A glutamine synthetase-like (GS-like) enzyme (NpaA1) initiates 1NA glutamylation, and this enzyme exhibits a broad substrate selectivity toward a variety of anilines and naphthylamine derivatives. During γ-glutamylation of 1NA, the 1NA consumption (0.16 mmol) was almost equivalent to the total accumulation of γ-glutamylated 1NA (0.157 mmol). In view of the above analyses, NpaA1 was established as a γ-glutamylnaphthylamide synthase catalyzing ligation of 1NA and L-glutamate to form γ-glutamylated 1NA. The crystal structure of apo-NpaA1 and two complexes with substrates or substrate analogs were obtained. The binding pocket is located at the interface between adjacent subunits, and the bifunnel channel similar to GS protein refers to a structural feature characterized by two distinct channels that converge into the common active site.

The model of NpaA1 built by Alphafold2 was used as the template for a molecular replacement for apo-NpaA1. The crystal structure of apo-NpaA1 revealed that there are six monomers arranged as a hexamer in an asymmetric unit. In apo NpaA1, there are two Mn2+ ions binding to the active center, coordinated by glutamic acid and histidine residues.

>[6x]WSHPQFEKENLYFQGMSRKFDFITKNNLWTNEQRDAADKVLAEIDSLGLEMIRLSWADQYGLLRGKSLTVASLKSAFKEGSEVAIGPFFFDLVSSMVFNLFTTAGDFEDELSGNPTVVMVPDPTTFKVLPWADKTGWMLADLHWKSGEPFPLCPRGIMKKAVKSLSDEGYLFKCGIELEWYLTKIVDRSLSPESLGAPGVQPDAIQVQPVAQGYSVLLEHHLDQVDDIMSKVRKGLLELNLPLRSIEDEWAPSQMETTFDVMEGLEAADAALLIKSAIKQICSRHGYHATFMCKPAINGFFASGWHMHQSLVDKDTRKNLFIPSEGEVLSPLGRAYAGGLLANGSAASSFTTPTVNGYRRRQPYSLAPDRRAWAKDNKAAMVRVVSATGDPASRIENRIGEPGANPYLYMASQIVSGLDGIKNKKDPGELQESPYDAQVPMLPTTLAEALDALEHDSELFRSCFGDTFIKYWLQLRRSEWARFLDAEGAEAAEPTGAVTQWEQKEYFNLL> AQSVPWGISRVQAPAAHNRGLTGSGVKVAVLDTGISTHPDLNIRGGASFVPGEPSTQDGNGHGTHVAGTIAALNNSIGVLGVAPSAELYAVKVLGASGSGSVSSIAQGLEWAGNNGMHVANLSLGSPSPSA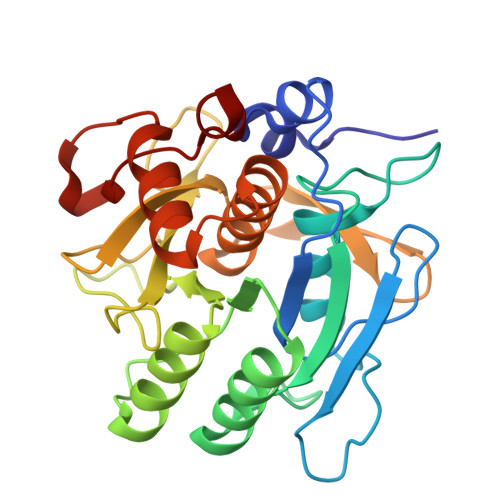TLEQAVNSATSRGVLVVAASGNSGAGSISYPARYANAMAVGATDQNNNRASFSQYGAGLDIVAPGVNVQSTYPGSTYASLNGTSMATPHVAGAAALVKQKNPSWSNVQIRNHLKNTATSLGSTNLYGSGLVNAEAATR>[3x]MLNPIVRKFQYGQHTVTLETGMMARQATAAVMVSMDDTAVFVTVVGQKKAKPGQDFFPLTVNYQERTYAAGRIPGSFFRREGRPSEGETLIARLIDRPIRPLFPEGFVNEVQVIATVVSVNPQVNPDIVAMIGASAALSLSGIPFNGPIGAARVGYINDQYVLNPTQDELKESKLDLVVAGTEAAVLMVESEAQLLSEDQMLGAVVFGHEQQQVVIQNINELVKEAGKPRWDWQPEPVNEALNARVAALAEARLSDAYRITDKQERYAQVDVIKSETIATLLAEDETLDENELGEILHAIEKNVVRSRVLAGEPRIDGREKDMIRGLDVRTGVLPRTHGSALFTRGETQALVTATLGTARDAQVLDELMGERTDTFLFHYNFPPYSVGETGMVGSPKRREIGHGRLAKRGVLAVMPDMDKFPYTVRVVSEITESNGSSSMASVCGASLALMDAGVPIKAAVAGIAMGLVKEGDNYVVLSDILGDEDHLGDMDFKVAGSRDGISALQMDIKIEGITKEIMQVALNQAKGARLHILGVMEQAINAPRGDISEFAPRIHTIKINPDKIKDVIGKGGSVIRALTEETGTTIEIEDDGTVKIAATDGEKAKHAIRRIEEITAEIEVGRVYTGKVTRIVDFGAFVAIGGGKEGLVHISQIADKRVEKVTDYLQMGQEVPVKVLEVDRQGRIRLSIKEATEQSQPAAAPEAPAAEQGE

Polynucleotide phosphorylase (PNPase) is an ancient exoribonuclease conserved in the course of evolution and is found in species as diverse as bacteria and humans. Although PNPase can catalyze the polymerization of nucleotides, its main cellular function is the 3ʹ-to-5ʹ degradation of RNA (Grunberg-Manago et al., 1955). While the catalytic core performs the phosphorolytic action, the KH and S1 domains participate in RNA substrate capture and autoregulation (Wong et al., 2013) and are powerful facilitators of PNPase activity. Cryoelectron microscopy (cryo-EM) was used to solve structures for E. coli PNPase in the apo- and substrate-bound forms and in a ternary complex with sRNA substrate and Hfq (i.e., the RNA carrier complex).

Structures of E. coli apo PNPase have been limited to the catalytic core and parts of the KH domains (Nurmohamed et al., 2009). A full structure has remained elusive, but it has been assumed to have flexibly tethered KH and S1 domains protruding outward from each PNPase protomer. The structure of E. coli PNPase in apo form reveals for the first time the wide conformational landscape of the KH and S1 RNA recognition modules.Recently, Ups1, a yeast member of the conserved mitochondrial intermembrane space (IMS) proteins, was shown to mediate PA transfer between the mitochondrial OM and IM in cooperation with Mdm35. Mdm35, another conserved yeast IMS protein, is a binding partner of Ups proteins, and facilitate their import into mitochondria. Surprisingly, two distinct polypeptides of Ups1 and Mdm35 form a single compact domain, the Ups1 part of which corresponds to the START (StAR-related lipid-transfer) domain, likely functioning as a lipid-binding domain. Like other START domain-containing proteins, the Ups1–Mdm35 complex contains a deep pocket that can accommodate a lipid molecule and an Ω-loop likely functioning as a lid for the pocket.

The full-length Ups1 (175 amino acids) and Mdm35 failed to cocrystallize, yet Ups1ΔC5 lacking the C-terminal five residues and Mdm35ΔC5 grew cocrystal. The crystal structure of the Ups1–Mdm35 complex was determined from its SeMet-labelled protein crystal by the single-wavelength anomalous dispersion method using the anomalous signal of selenium atoms, and was subsequently refined to 1.40-Å resolution against the data set from the native crystal. The asymmetric unit of the crystal contains two Ups1–Mdm35 heterodimers, which have a similar conformation to each other, with root mean square (r.m.s.) differences of 0.6 and 0.3 Å for 168 and 72 Cα atoms of Ups1 and Mdm35, respectively. In the asymmetric unit, two Ups1 molecules were found to form a domain-swapped dimer; the two Ups1 molecules exchange the identical C-terminal helix (residues 135–170) each other. Therefore, the domain-swapped conformation likely arose from the crystallization artifact, and we thus refer to the monomeric Ups1–Mdm35 heterodimer, in which the C-terminal segment is connected to the polypeptide of the remaining part in the same molecule, as the Ups1–Mdm35 complex. Ups1 contains two α-helices (α1 and α2) and a seven-stranded antiparallel β-sheet, which is folded into a half-barrel structure (β1-β7) and an Ω-loop (Ω1, residues 62–71) is formed between the β3 and β4 strands. Like free Mdm35, Mdm35 in the complex with Ups1, takes an antiparallel α-hairpin (α1 and α2), yet the C-terminal segment, which is disordered in free Mdm35, forms an α-helix (α3). Mdm35 embraces Ups1 with the three α helices, covering ∼1,400 Å2 (12% of the total surface area of the Ups1 molecule), rendering the Ups1–Mdm35 complex folded into a single-domain like structure. A closer look at the crystal structure of the Ups1–Mdm35 complex indicates that the hydrophobic side chains of Tyr20, Phe24, Trp27, Tyr28 and Phe32 in the α1 helix and Trp46 and Tyr49 in the α2 helix of Mdm35 bind to the hydrophobic region formed by Phe15, Ser19, Phe23, Thr39, Arg42, Leu50, Val84 and Pro86 of Ups1. The entrance of the pocket is nearly closed by the Ω1 loop.

>MGNIMSASFAPECTDLKTKYDSCFNEWYSEKFLKGKSVENECSKQWYAYTTCVNAALVKQGIKPALDEAREEAPFENGGKL[2x];>[2x]MGSSHHHHHHSQDPMVLLHKSTHIFPTDFASVSRAFFNRYPNPYSPHVLSIDTISRNVDQEGNLRTTRLLKKSGKLPTWVKPFLRGITETWIIEVSVVNPANSTMKTYTRNLDHTGIMKVEEYTTYQFDSATSSTIADSRVKFSSGFNMGIKSKVEDWSRTKFDENVKKSRMGMAFVIQKLEEA6-chloro-4-phenyl-2-(piperidin-1-yl)-3-(1H-tetrazol-5-yl)quinoline | C21 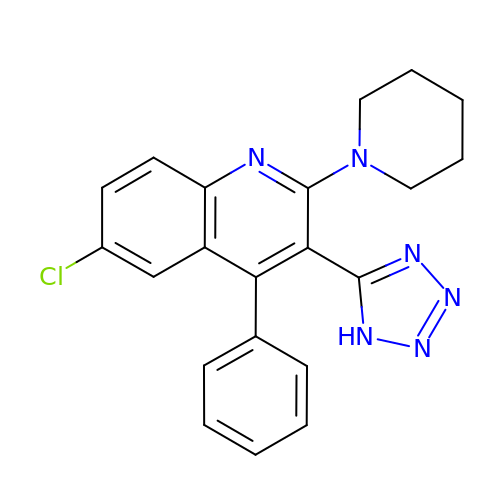H19 Cl N6 | FXEKONNOBJEKPB-UHFFFAOYSA-N>MERPQPDSMPQDLSEALKEATKEVHTQAENAEFMRNFQKGQVTRDGFKLVMASLYHIYVALEEEIERNKESPVFAPVYFPEELHRKAALEQDLAFWYGPRWQEVIPYTPAMQRYVKRLHEVGRTEPELL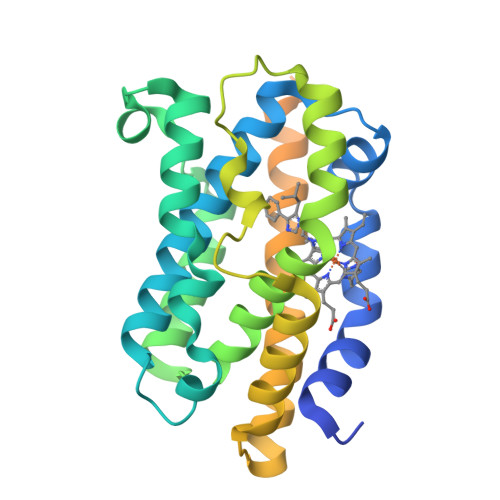VAHAYTRYLGDLSGGQVLKKIAQKALDLPSSGEGLAFFTFPNIASATKFKQLYRSRMNSLEMTPAVRQRVIEEAKTAFLLNIQLFEELQELLTHDTKDQSPSRAPGLRQRASNKVQDSAPVETPRGKPPLNTRSQAPLLRWVLTLSFLVATVAVGLYAM[2x]> TITVSTPIKQIFPDDAFAETIKANLKKKSVTDAVTQNELNSIDQIIANNSDIKSVQGIQYLPNVRYLALGGNKLHDISALKELTNLGWLNLSNNQLETLPQGVFEKLTNLTTLNLSNNQLTSLPQGVFERLASLTTLNLSNNQLTSLPQGVFERLTNLTTLNLSNNQLTSLPQGVFERLTNLTTLNLSNNQLTSLPQGVFERLTSLHTLDLSNNGITDISALKNLDNLHTLDLSNNGITDIS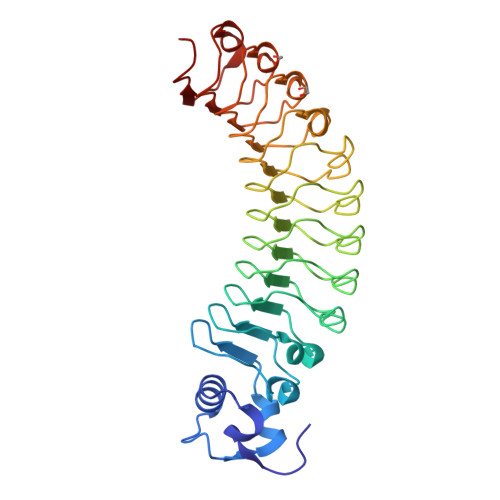ALKNLDNLHTLDLSNNGITDISALKNLTSLHTLDLSNNGITDISALKNLDNLETLDLRNNGI>DDATADSRKTYTLTDYLKNTYRLKLYSLRWISDHEYLYKQENNILVFNAEYGNSSVFLENSTFDEFGHSINDYSISPDGQFILLEYNYVKQWRHSYTASYDIYDLNKRQLITEERIPNNTQWVTWSPVGHKLAYVWNNDIYVKIEPNLPSYRITWTGKEDIIYNGITDWVYEEEVFSAYSALWWSPNGTFLAYAQFNDTEVPLIEYSFYSDESLQYPKTVRVPYPKAGAVNPTVKFFVVNTDSLSSVTNATSIQITAPASMLIGDHYLCDVTW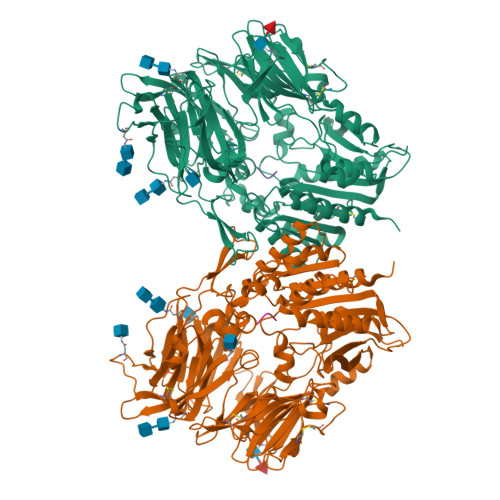ATQERISLQWLRRIQNYSVMDICDYDESSGRWNCLVARQHIEMSTTGWVGRFRPSEPHFTLDGNSFYKIISNEEGYRHICYFQIDKKDCTFITKGTWEVIGIEALTSDYLYYISNEYKGMPGGRNLYKIQLSDYTKVTCLSCELNPERCQYYSVSFSKEAKYYQLRCSGPGLPLYTLHSSVNDKGLRVLEDNSALDKMLQNVQMPSKKLDFIILNETKFWYQMILPPHFDKSKKYPLLLDVYAGPCSQKADTVFRLNWATYLASTENIIVASFDGRGSGYQGDKIMHAINRRLGTFEVEDQIEAARQFSKMGFVDNKRIAIWGWSYGGYVTSMVLGSGSGVFKCGIAVAPVSRWEYYDSVYTERYMGLPTPEDNLDHYRNSTVMSRAENFKQVEYLLIHGTADDNVHFQQSAQISKALVDVGVDFQAMWYTDEDHGIASSTAHQHIYTHMSHFIKQCFSLPHHHHHH[2x];>IPI[2x]> GPLEDQEEN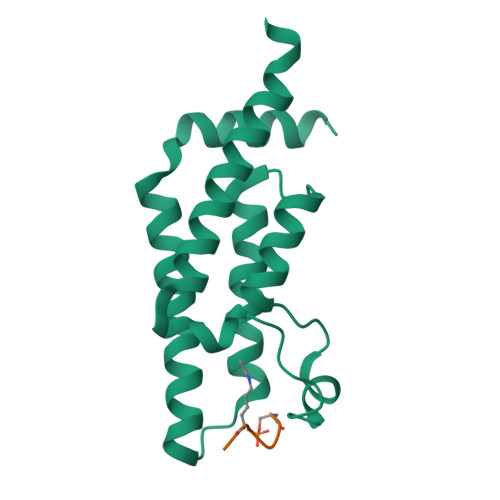TLRELRLFLRDVTKRLATDKRFNIFSKPVDIEEVSDYLEVIKEPMDLSTVITKIDKHNYLTAKDFLKDIDLICSNALEYNPDKDPGDKIIRHRACTLKDTAHAIIAAELDPEFNKLCEEIKEARIKR;> SGRGKGGKGLGKGG> DSLSKSPENWMSKLDDGKHLTEINIPGSHDSGSFTLKDPVKSVWAKTQDKDYLTQMKSGVRFFDIRGRASADNMISVHHGMVYLHHELGKFLDDAKYYLSAYPNETIVMSMKKDYDSDSKVTKTFEEIFREYYYNNPQYQNLFYTGSNANPTLKETKGKIVLFNRMGG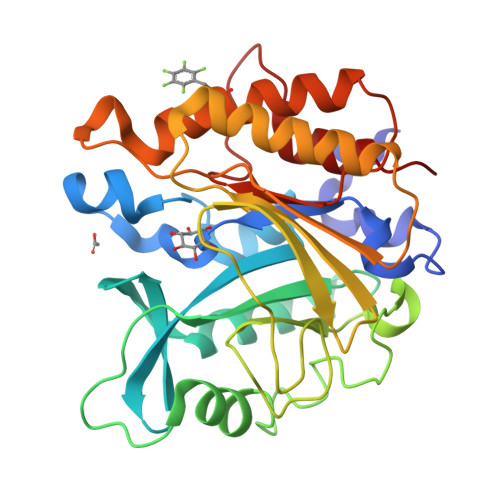TYIKSGYGADTSGIQWADNATFETKINNGSLNLKVQDEYKDYYDKKVEAVKNLLAKAKTDSNKDNVYVNFLSVASGGSAFNSTYNYASFINPEIAKTIKANGKARTGWLIVDYAGYTWPGYDDIVSEIIDSNKL(5S)-3-methyl-7-(trifluoromethyl)pyrrolo[1,2-a]pyrazin-1(2H)-one 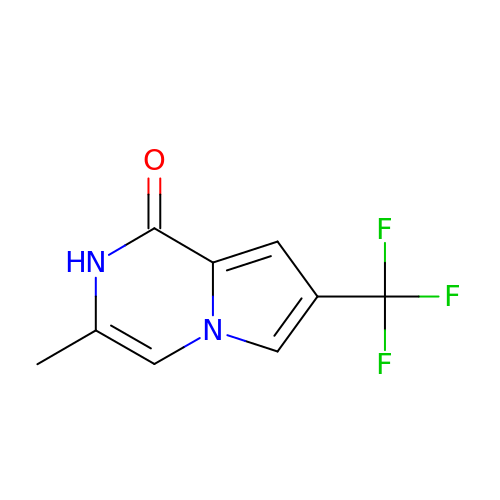| C9 H7 F3 N2 O | DYHQRCYZMPRXNH-UHFFFAOYSA-N>[4x]MAAGVAAW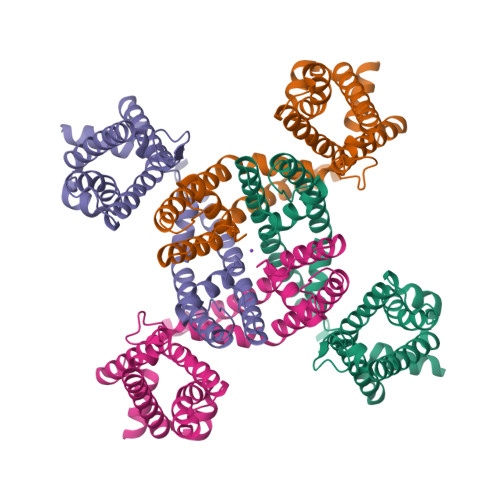LPFARAAAIGWMPVASGPMPAPPRQERKRTQDALIVLNVSGTRFQTWQDTLERYPDTLLGSSERDFFYHPETQQYFFDRDPDIFRHILNFYRTGKLHYPRHECISAYDEELAFFGLIPEIIGDCCYEEYKDRRRENAERLQDDADTDTAGESALPTMTARQRVWRAFENPHTSTMALVFYYVTGFFIAVSVIANVVETVPCGSSPGHIKELPCGERYAVAFFCLDTACVMIFTVEYLLRLAAAPSRYRFVRSVMSIIDVVAILPYYIGLVMTDNEDVSGAFVTLRVFRVFRIFKFSRHSQGLRILGYTLKSCASELGFLLFSLTMAIIIFATVMFYAEKGSSASKFTSIPAAFWYTIVTMTTLGYGDMVPKTIAGKIFGSICSLSGVLVIALPVPVIVSNFSRIYHQNQRADKRRAQKKARLARIRAAKSGSANAYMQSKRNGLLSNQLQSSEDEQAFVSKSGSSFETQHHHLLHCLEKTTNHEFVDEQVFEESCMEVATVNRPSSHSPSLSSQQG>QTDVIAQRKAILKQMGEATKPIAAMLKGEAKFDQAVVQKSLAAIADDSKKLPALFPADSKTGGDTAALPKIWEDKAKFDDLFAKLAAAATAAQGTIKDEASLKANIGGVLGNCKSCHDDFRAKKS[2x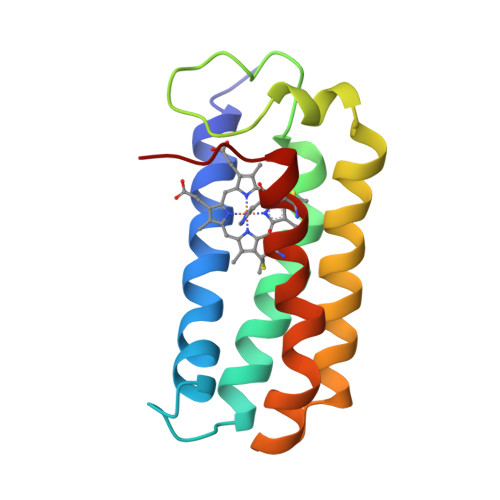]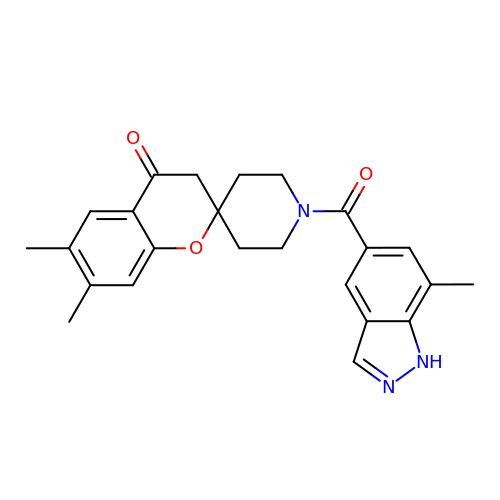6,7-dimethyl-1'-[(7-methyl-1H-indazol-5-yl)carbonyl]spiro[chromene-2,4'-piperidin]-4(3H)-one | C24 H25 N3 O3 | PQQBCUZITMWICX-UHFFFAOYSA-N Legionella pneumophila, the causative agent of Legionnaires disease, secretes the enzyme AnkX that uses cytidine diphosphate-choline to post-translationally modify the human small G-Protein Rab1 with a phosphocholine moiety at Ser76. Later in the infection, the Legionella enzyme Lem3 acts as a dephosphocholinase, hydrolytically removing the phosphocholine. Through crystal structures of Lem3 in the apo form and in complex with Rab1b, we reveal Lem3’s catalytic mechanism, showing that it acts on Rab1 by locally unfolding it. Since Lem3 shares high structural similarity with metal-dependent protein phosphatases, our Lem3:Rab1b complex structure also sheds light on how these phosphatases recognise protein substrates.

Therefore, we used a site-specific covalently linking strategy to capture the Lem3:Rab1b complex. Size exclusion chromatography and SDS-PAGE gel shift analysis demonstrated that the purified complex Lem3C134S_C209S_T391C_C395S_C456S:Rab1bS76T(PC-C3) (referred to as complexT391C) was present as a pure monomeric species. Furthermore, as demonstrated for Lem3 wildtype, the mutants cannot demodify Rab1bS76T(PC), permitting us to obtain a stable complex. Crystals of complexT391C diffracted to 2.15 Å and hence permitted its structure determination. No specific interactions are visible for the C3 linker region while L68Lem3 shows hydrophobic interaction with the choline group. The phosphate moiety of the linker in complexT391C does not participate in direct interactions with amino acids, but is involved in the coordination of three metal ions located in the active centre of Lem3 at the same site as observed in the Lem321-486 structure and coordinated by the same residues (D105Lem3, D254Lem3, and D394Lem3, D105Lem3 and G106Lem3). In addition, a third metal ion (M3) can be placed in the electron density, which is coordinated by D254Lem3 and D190Lem3. Rab1b:GDP binds to the hollow region of Lem321-486. As a consequence, the sequence R71-T74Rab1b of switch II is reorganized into a β-strand (β’β3-4,Rab1b) and placed between the β-hairpin (located on top of the fist) and the thumb. F215Lem3 occupies the position of Y78Rab1b, which is located in the hydrophobic pocket in the Rab1b-apo-structure. As a consequence, Y78Rab1b is displaced by 9.9 Å (distance between Cα-atoms), likely contributing to the movement of switch II towards Lem3’s active centre.

> GHMDKIITGKKIIFSQSVAKDQTKNLSSFLSERFYSVNQSHNHSIIIGSSLSHQENDIEHDTILDTSGVLVTTDTNGIVNGARVAITDGLGGGNGDQEEDDEIYRVSHSSCENFLNSDQNIDTTLSLITQPKASDKKQTAPKTLQHTEASMAAFIYQNHPGKGYIGEFANIGDGLIIILDKRFKIKHMVSASHIYRGFGTWTPPSLQALATTANKDALLVRQTLKLAEGDIIISMTDGVWGELKTSLIAQTNDRRDIGVDKEYFKTLFDELTDAPYPSSFDIARIITQRAMSRSLERRKTLIKLINEIEQQHFHEKSVKTINEVLEYFIKTGHVETAQTLKAILFEDGLSDGITYFENIEIPLEMVMHDLKSRCVGDCSTINVTRIPYHLDELIRGFINYPEKHQILAPLFKARVKSEADLEEAFHRLSLEMVQPEIESPISETHFERAFKKETLDKTQAVLTHYFRIS;> GPMPEYDYLFKLLLIGDSGVGKSCLLLRFADDTYTESYISTIGVDFKIRTIELDGKTIKLQIWDTAGQERFRTITSTYYRGAHGIIVVYDVTDQESYANVKQWLQEIDRYASENVNKLLVGNKSDLTTKKVVDNTTAKEFADSLGIPFLETSAKNATNVEQAFMTMAAEIKKRMG1-BETA-RIBOFURANOSYL-1,3-DIAZEPINONE 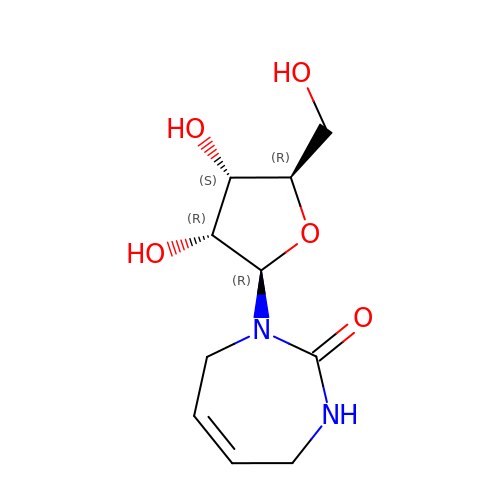| C10 H16 N2 O5 | HBBIVXDEBCKFIZ-FNCVBFRFSA-N2-(5-chloro-2-methylphenyl)-1-methyl-5-(2-{[4-(4-methylpiperazin-1-yl)phenyl]amino}pyrimidin-4-yl)-1H-pyrrole-3-carboxamide 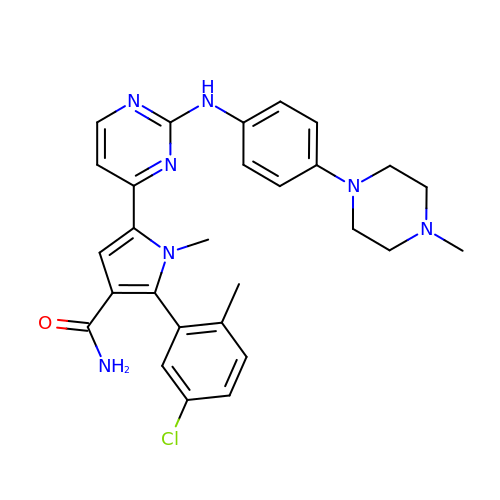| C28 H30 Cl N7 O | GTPKZTQLTICGMS-UHFFFAOYSA-N> MGELFRSEEMTLAQLFLQSEAAYCCVSELEELGKVQFRDLNPDVNVFQRKFVNEVRRCEEMDRKLRFVEKEIRKANIPIMDTGENPEVPFPRDM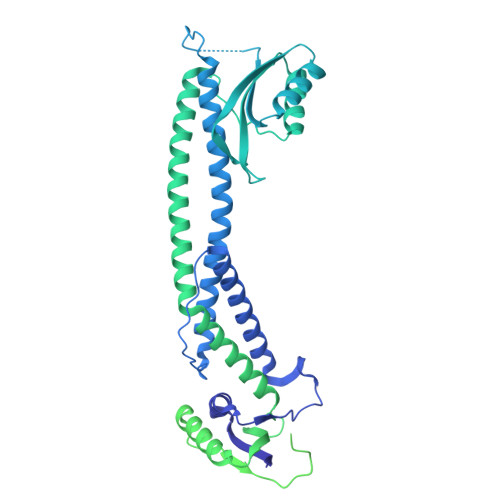IDLEANFEKIENELKEINTNQEALKRNFLELTELKFILRKTQQFFDEMADPDLLEESSSLLEPNEMGRGAPLRLGFVAGVINRERIPTFERMLWRVCRGNVFLRQAEIENPLEDPVTGDYVHKSVFIIFFQGDQLKNRVKKICEGFRASLYPCPETPQERKEMASGVNTRIDDLQMVLNQTEDHRQRVLQAAAKNIRVWFIKVRKMKAIYHTLNLCNIDVTQKCLIAEVWCPVTDLDSIQFALRRGTEHSGSTVPSILNRMQTNQTPPTYNKTNKFTHGFQNIVDAYGIGTYREINPAPYTVITFPFLFAVMFGDFGHGILMTLFAVWMVLRESRILSQKNENEMFSMVFSGRYIILLMGLFSIYTGLIYNDCFSKSLNIFGSSWSVRPMFTIGNWTEETLLGSSVLQLNPAIPGVFGGPYPFGIDPIWNIATNKLTFLNSFKMKMSVILGIIHMLFGVSLSLFNHIYFKKPLNIYFGFIPEIIFMSSLFGYLVILIFYKWTAYDAHSSRNAPSLLIHFINMFLFSYPESGNAMLYSGQKGIQCFLIVVAMLCVPWMLLFKPLILRHQYLRKKHLGTLNFGGIRVGNGPTEEDAEIIQHDQLSTHSEDAEEPTEDEVFDFGDTMVHQAIHTIEYCLGCISNTASYLRLWALSLAHAQLSEVLWTMVIHIGLHVRSLAGGLGLFFIFAAFATLTVAILLIMEGLSAFLHALRLHWVEFQNKFYTGTGFKFLPFSFEHIREGKFDE>MERKHHFVLVHNACHGAWIWYKLKPLLESAGHRVTAVELAASGIDPRPIQAVETVDEYSKPLIETLKSLPENEEVILVGFSFGGINIALAADIFPAKIKVLVFLNAFLPDTTHVPSHVLDKLMEMFGGWGDTEFSSHETRNGTMSLLKMGPKFMKARLYQNCPIEDYELAKMLHRQGSLFTEDLSKKEKFSEEGYGSVQRVYVMSSEDKIIPCDFIRWMIDNFNVSKVYEI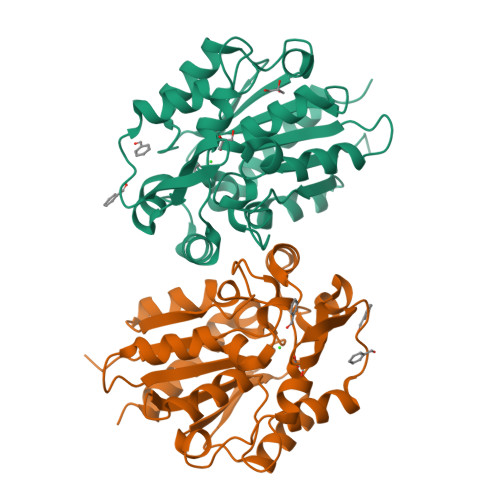DGGDHMVMLSKPQKLFDSLSAIATDYMGL[2x]>DSEDEFPEITEEMEKEIKNVFRNGNQDEVLSEAFRLTITRKDIQTLNHLNWLNDEIINFYMNMLMERSKEKGLPSVHAFNTFFFTKLKTAGYQAVKRWTKKVDVFSVDILLVPIHLGVHWCLAVVDFRKKNITYYDSMGGINNEACRILLQYLKQESIDKKRKEFDTNGWQLFSKKSQEIPQQMNGSDCGMFACKYADCITKDRPI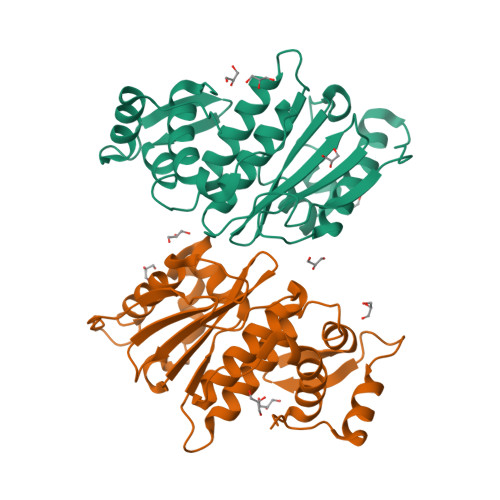NFTQQHMPYFRKRMVWEILHRKLL[2x]> HHHHHHGSSPKEEKFKKKLEEELKKIRERLLMVFDEERVEEYMKIMKEVIEKILENRKKGSKEKVEIPPGMEWFYENFLRYYD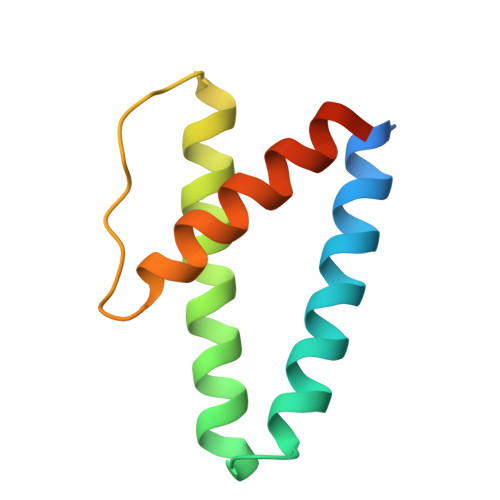YEEEKLEKEEKE> MQNHSQEQVNLKVGEVVQYLLIKDQKKLPIKRADIVRSVIKEYKDIYPEIIHRAQITLQQVFGFQLE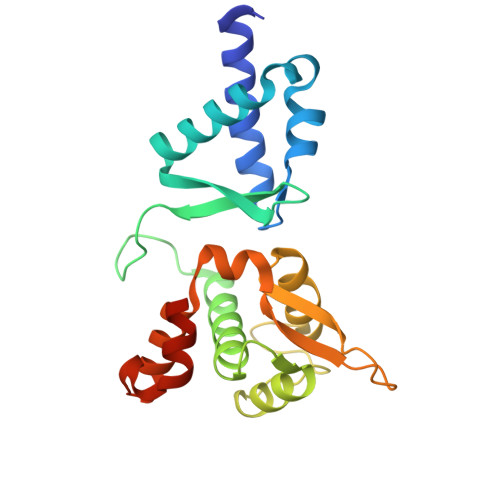EIDTKSHIYILTNKLQRVQGDGMRVDENTSKLGLLMVILSLIFMKGNTAKESAIWEMLRRLRIEPGEMHSEFGDVKKLVTEEFVKQKYLEYNKVPHIDPVEYEFRWGQRAFKETSKMKVLEFVSKIQQKDPKSWTTQYKDAQEQTQVAGR> AMADLEQKVLEMEASTYDGVFIWKISDFARKRQEAVAGRIPAIFSPAFYTSRYGYKMCLRIYLNGDGTGRGTHLSLFFVVMKGPNDALLRWPFNQKVTLMLLDQNNREHVIDA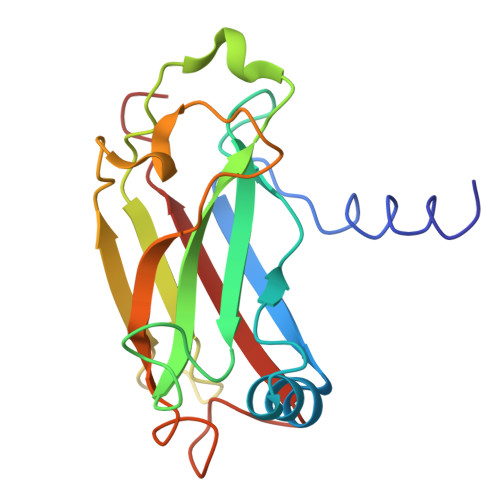FRPDVTSSSFQRPVNDMNIASGCPLFCPVSKMEAKNSYVRDDAIFIKAIVDLTGL>[2x]GPLGMATEEAIIRIPPYHYIHVLDQNSNVSRVEVGPKTYIRQDNERVLFAPVRMVTVPPRHYCIVANPVSRDAQSSVLFDV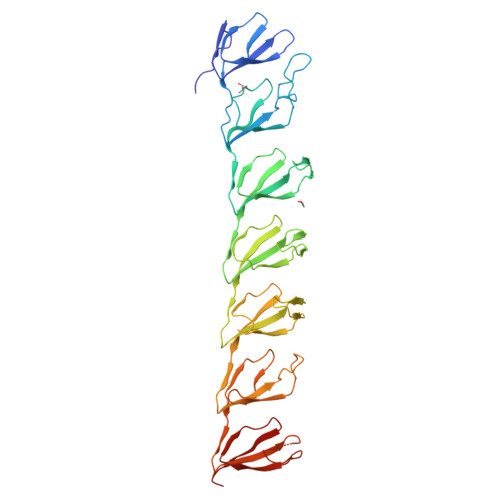TGQVRLRHADQEIRLAQDPFPLYPGELLEKDITPLQVVLPNTALHLKALLDFEDKNGDKVMAGDEWLFEGPGTYIPQKEVEVVEIIQATVIKQNQALRLRARKECFDRDGKERVTGEEWLVRSVGAYLPAVFEEVLDLVDAVILTEKTALHLRARQNFKDLRGVAHRTGEEWLVTVQDTEAHVPDVYEEVLGVVPITTLGPRHYCVILDPMGPDGKNQLGQKRVVKGEKSFFLQPGERLERGIQDVYVLSEQQGLLLKALQPLEEGEGEERVAHQAGDRWLIRGPLEYVPSAKVEVVEERQAIPLD>[3x]QDDASDRQTREVLDPIVASLMEAQQIPGMAIALVRPEGTTISHYGAADRETGTPVDDDTLFEIGSLSKTLTATLASLAEVEGKLDFDAPVSRYLPELEGSAFDDISGLNLGTHTGGGLPLFVPDEVTDRASLMAWYREWQPTEPIGESRTYSN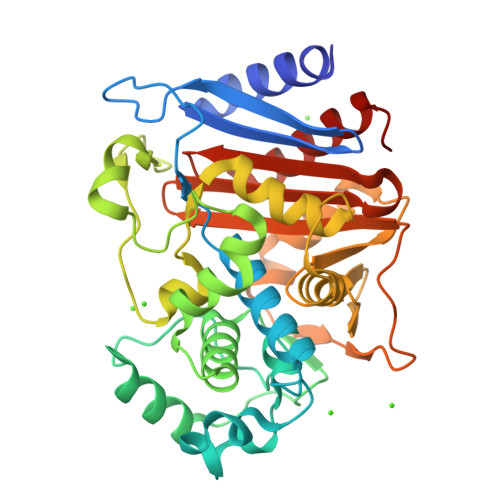LGIGLLGLETAASLDGEFVPTMRAKVLAPLGMQDTWYDVPEARMADYAMGEDKDGQPTRVSPGVLDDEAYGIKTTAADLAKLVRANLHLADVDAELQQAIDATRQGHYRVGDMTQALIWEQYSLPVAPETLRAGQGYDMILEPNAAEALEPPQSPRDDVWVNKTGSTQGFGGYIVMLPGKHTGLVMLANKNYPNDARVEAAYRILSGLGAIDVP>[2x]GSRLETEIERCRSECQWERIPELVKQLSAKLIANDDMAELLLGESKLEQYLKEHPLRQGASPRGPKPQLTEVRKHLTAALDRGNLKSEFLQESNLIMAKLNYVEGDYKEALNIYARVGLDDLPLTAVPPYRLRVIAEAYATKGLCLEKLPISSSTSNLHVDREQDVITCYEKAGDIALLYLQEIERVILSNIQNRSPKPGPAPHDQELGFFLETGLQRAHVLYFKNGNLTRGVGRFRELLRAVETRTTQNLRMTIARQLAEILLRGMCEQSYWNPLEDPPCQSPLDDPLRKGANTKTYTLTRRARVYSGENIFCPQENTEEALLLLLISESMANRDAVLSRIPEHKSDRLISLQSASVVYDLLTIALGRRGQYEMLSECLERAMKFAFEEFHLWYQFALSLMAAGKSARAVKVLKECIRLKPDDATIPLLAAKLCMGSLHWLEEAEKFAKTVVDVGEKTSEFKAKGYLALGLTYSLQATDASLRGMQEVLQRKALLAFQRAHSLSPTDHQAAFYLALQLAISRQIPEALGYVRQALQLQGDDANSLHLLALLLSAQKHYHDALNIIDMALSEYPENFILLFSKVKLQSLCRGPDEALLTCKHMLQIWKSCYNLTNPSDSGRGSSLLDRTIADRRQLNTITLPDFSDPETGSVHATSVAASRVEQALSEVASSLQSSAPKQGPLHPWMTLAQIWLHAAEVYIGIGKPAE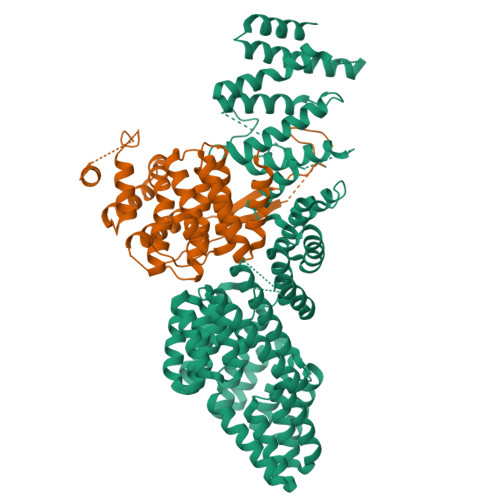ATACTQEAANLFPMSHNVLYMRGQIAELRGSMDEARRWYEEALAISPTHVKSMQRLALILHQLGRYSLAEKILRDAVQVNSTAHEVWNGLGEVLQAQGNDAAATECFLTALELEASSPAVPFTIIPRVL;>[2x]GPLGSFTSEKGVVEEWLSEFKTLPETSLPNYATNLKDKSSLVSSLYKVIQEPQSELLEPVCHQLFEFYRSGEEQLLQFTLQFLPELIWCYLAVSASRNVHSSGCIEALLLGVYNLEIVDKQGHTKVLSFTIPSLSKPSVYHEPSSIGSMALTESALSQHGLSKVVYSGPHPQREMLTAQNRFEVLTFLLLCYNAALTYMPSVSLQSLCQICSRICVCGYPRQHVRKYKGISSRIPVSSGFMVQMLTGIYFAFYNGEWDLAQKALDDIIYRAQLELYPEPLLVANAIKASLPHGPMKSNKEGTRCIQVEITPT>MGSRVAHRNTSGCPVNCVVSRPALGRNPLACLIHGLALGLSLTQAGAALAADGDTDQDHALTLDTSVISATQPDSATGPQAGYVAKRSLSGTKTDASLSEIPQSISVITRDQMDAQQVQSVNEALRYTAGVQANTTAASQRFDTLSIRGF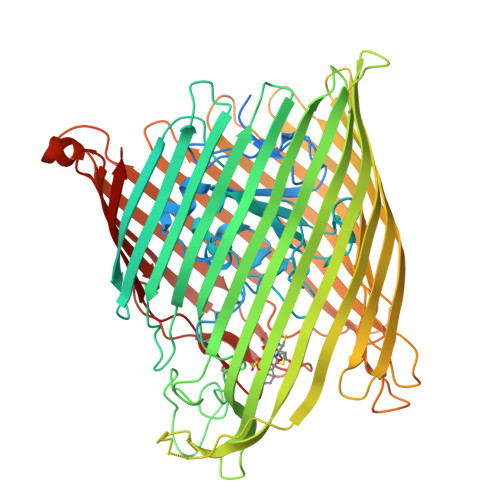DVTTGMLRDGLKGNTAQAWPKVEAYGLERIDVLKGPASVLFGQNSPGGVVNQISKRPLDKPFHEVQIQGGSFDRAQGQFDFSGPLDDEGQFLYRLVGLERDSGTQFDHIKDDKQYFAPSFTWKPNDDTSLTLLADYTQDTFGAPRVFLPAQGTLLGNPNGKVRHNVFLDEPGLDNDRTQYSLGYLLEHRLNDVWSLNSSARYGHVNLLTNTASGMSLAPDLRTLNRAAYRFRIVGDTYSLDNNAQARWNLGSTQMVSLLGIDYRRTREDYYLRGGSASPIDIYNPVHHHHHHGGVFDPSTPFTNTVQRADQVGVYAQQQFTFDEHWVLTVGGRQDRSSARTDNRMNDSGSKQDDEKFTYRTGLVYLADNGLAPYISYSTSFDPVLGTNFYGTPYKPTSAKQSEVGVKYQPPGIDSYITLSLFDLTQENVLTTDPAQRLNKIQTGEINVRGIELEGKASLARGLDLLAALTYNDAEVSKSNNPLEKGKRPTDTPEKMASLWADYTLPEGPLSGLGFGAGVRYIGSTEADAANTQRVPSYTLLDAAVHYDFDKLIPAAKGLRLAVNATNLTDKHYYEGCSLTNCSAGYDRSVIASLRYRW[2x]>GPMEPRSMEYFCAQVQQKDVGGRLQVGQELLLYLGAPGAISDLEEDLGRLGKTVDALTGWVGSSNYRVSLMGLEILSAFVDRLSTRFKSYVAMVIVALIDRMGDAKDKVRDEAQTLILKLMDQVAPPMYIWEQLA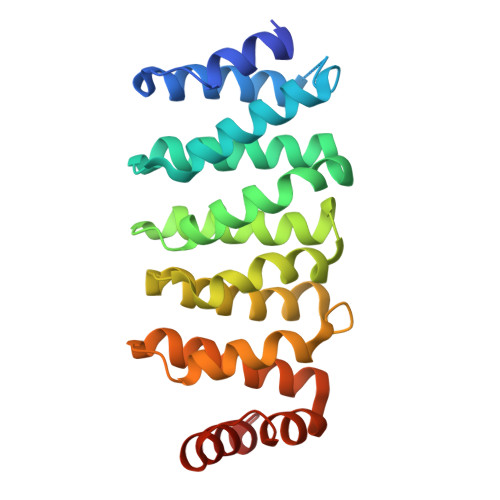SGFKHKNFRSREGVCLCLIETLNIFGAQPLVISKLIPHLCILFGDSNSQVRDAAILAIVEIYRHVGEKVRMDLYKRGIPPARLEMIFAKFDEVQS[2x]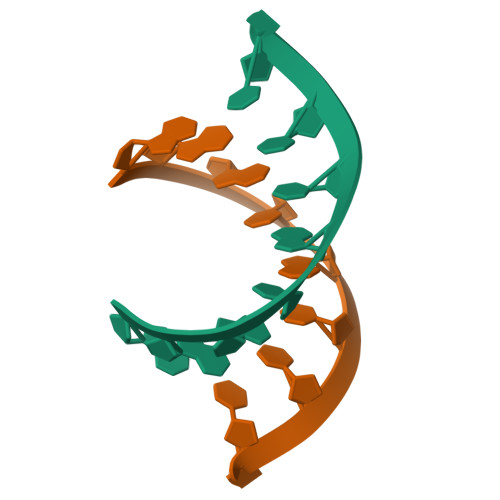>[2x]GGGCGCUCC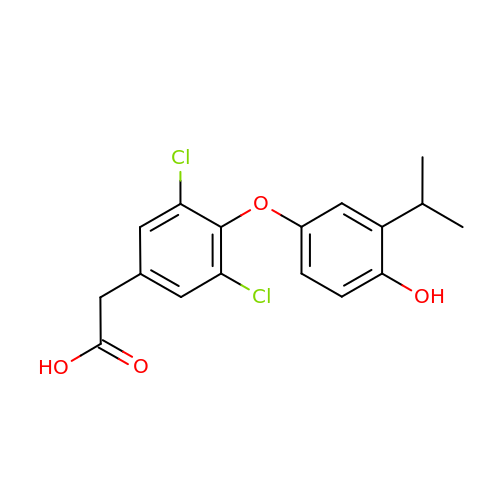{3,5-DICHLORO-4-[4-HYDROXY-3-(PROPAN-2-YL)PHENOXY]PHENYL}ACETIC ACID | C17 H16 Cl2 O4 | OZYQIQVPUZANTM-UHFFFAOYSA-N2,2'-[thiophene-2,5-diyldi(4,1-phenylene)]diacetic 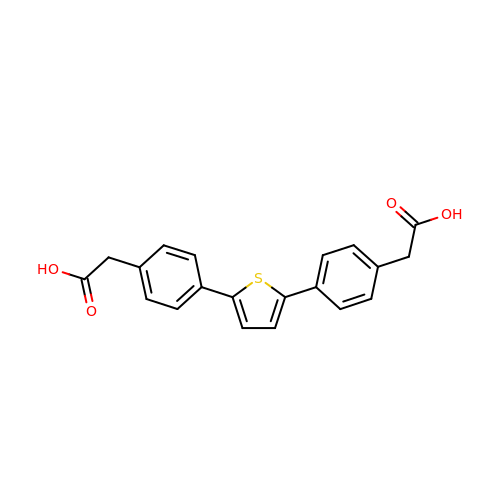acid | C20 H16 O4 S | ZDYJCKHDQKYXFY-UHFFFAOYSA-N Sterile alpha motif and HD domain-containing protein 1 (SAMHD1) is an important regulator of cellular 2′-deoxynucleoside-5′-triphosphate (dNTP) in mammalian cells. Although the HD-domain contains the active site, dNTP hydrolysis requires assembly of SAMHD1 into homo-tetramers. Here, sequences at the N and C termini of the HD-domain stabilise inter-monomer protein–protein interactions and incorporate four pairs of allosteric nucleotide-binding sites, AL1 and AL2, which regulate the enzyme through combined binding of G-based (AL1) and 2′-deoxynucleoside (AL2) triphosphates. Using combined biophysical and X-ray structural studies incorporating nucleotide analogues along with mutagenesis experiments we have now discovered that SAMHD1 uses a bi-metallic Fe–Mg centre to catalyse dNTP hydrolysis in a reaction similar to those catalysed by HD domains in both human and bacterial phosphodiesterase PDE enzymes.

In addition, we determined the structures of two co-complexes of wt-SAMHD1(109-626), also in the presence of Mg2+, with (i) GTP (AL1), dATP (AL2) and dCMPNPP (active site) and (ii) GTP (AL1), dATP (AL2) and TMPNPP (active site). dATP was added to the latter two complexes to stimulate tetramer assembly, as dCMPNPP and TMPNPP are poor AL2 activators. SEC-MALLS analysis revealed that all four dNMPNPP analogues, which have an imido substitution at the α,β-bridging oxygen, when combined with GTP, support the formation of stable SAMHD1 tetramers, albeit to varying degrees. Near-complete tetramerisation was observed with dAMPNPP, while dCMPNPP promoted the least tetramerisation and dGMPNPP was able to support tetramerisation without additional GTP, presumably by occupying both AL1 and AL2 allosteric sites. The most significant effect of dATP addition was observed with dCMPCPP, with kcat being increased 2.5-fold, presumably due to the limited ability of C-based nucleotides to induce SAMHD1 tetramerisation by AL2 binding. Further investigation using inhibition assays revealed that all dNMPNPP analogues were actually competitive inhibitors of SAMHD1-dNTP triphosphohydrolase activity, with inhibition constants (Ki) ranging from 0.78 µM for dAMPNPP to 0.052 µM for dGMPNPP, with the following rank order of increasing affinity: dAMPNPP < TMPNPP < dCMPNPP < dGMPNPP. The resolution of these structures varied between 2.0 and 3.2 Å, but all structures contain highly homologous “closed” tetramers of the SAMHD1 catalytic domain, with pairwise root-mean-square deviations (RMSDs) of <0.5 Å across all atoms in each tetramer. In the active site of the dNMPNPP structures, regardless of the nucleotide base, it is apparent that the side chain of Asp311 of the HD motif not only makes a coordinate bond with the bound active site Fe but also acts as an acceptor in a hydrogen bonding interaction with the proton (Himido) of the α,β-imido group of the dNMPNPP.

>[16x]GSQIHVDTMKVINDPIHGHIELHPLLVRIIDTPQFQRLRYIKQLGGGYYVFPGASHNRFEHSLGVGYLAGCLVHALGEKQPELQISERDVLCVQIAGLCHDLGHGPFSHMFDGRFIPLARPEVKWTHEQGSVMMFEHLINSNGIKPVMEQYGLIPEEDICFIKEQIVGPLESPVEDSLWPYKGRPENKSFLYEIVSNKRNGIDVDKWDYFARDCHHLGIQNNFDYKRFIKFARVCEVDNELRICARDKEVGNLYDMFHTRNSLHRRAYQHKVGNIIDTMITDAFLKADDYIEITGAGGKKYRISTAIDDMEAYTKLTDNIFLEILYSTDPKLKDAREILKQIEYRNLFKYVGETQPTGQIKIKREDYESLPKEVASAKPKVLLDVKLKAEDFIVDVINMDYGMQEKNPIDHVSFYCKTAPNRAIRITKNQVSQLLPEKFAEQLIRVYCKKVDRKSLYAARQYFVQWCADRNFTKPQDGDVIAPLITPQKKEWNDSTSVQNPTRLREASKSRVQLFKDDPM>[4x]SMGPTSQRRGSLQLWQFLVALLDDPSNSHFIAWTGRGMEFKLIEPEEVARRWGIQKNRPAMNYDKLSRSLRYYYEKGIMQKVAGERYVYKFVCDPEALFSMAFSDN

The Ets transcription factor family consists of 28 genes in humans containing the evolutionarily conserved 85 amino acid Ets DNA-binding domain, originally identified as a viral oncogene (E26 transformation-specific). The Ets domain is a variant helix-turn-helix (winged helix) structure, comprising three α-helices and a four-stranded antiparallel β-sheet. Here, we present the crystal structures of the Ets domains of the entire PEA3 subfamily (Etv1, Etv4, and Etv5) together with the structure of the Erg family member (Fev). Furthermore, a new Ets dimerization interface linked by a redox-sensitive disulfide bond is identified, and this dimerization is shown to result in a significant inhibition of DNA binding, potentially linking Ets transcription factors with cellular redox regulatory mechanisms.

Crystals were obtained from constructs that contained the Ets domain, Etv1 (encompassing amino acids 326–429), Etv4 (encompassing amino acids 338–470), and Fev (encompassing amino acids 42–141). The construct of Etv1 included two inadvertent mutations that resulted from primer impurities as follows: Y329S at the N terminus, and P427S at the C terminus; this construct is denoted Etv1Y329S-P427S. Our attempts to crystallize the corresponding construct with the wild-type sequence failed, although the mutated residues are in disordered regions or at the end of the ordered region of the crystal structures of Etv1, so they are unlikely to have any bearing on the structural and functional analyses. Electron density is observed for residues Ser-334 to Phe-426 (thus excluding the Y329S and P427S mutations) with most side chains visible. We also compared the Etv-1 construct used for crystallization, which contains two primer-induced mutations, against wild-type Etv1 and found no significant difference in DNA binding. Etv1, Etv4, and Fev display the typical fold of the Ets domain, which contains three α-helices (α1–3) flanking a four-stranded β-sheet, with an additional C-terminal helix (α4). On an individual residue level, the most striking transitions can be seen to occur in the recognition helix α3, where in Etv1 Asp-387, Arg-391, and Arg-394 can be seen to become ordered upon DNA binding and Tyr-395, which can be seen to switch between the two alternative rotamers found to be important for recognition of bases downstream of the GGA motif in the Fev-DNA complex. Analysis of the contacts between adjacent molecules in the Etv1, Etv4, and Etv5 crystals reveals a conserved potential dimer interface that is distant from the DNA binding surface and is present in all the DNA-free and DNA-bound crystal forms. Dimerization of Etv1, -4, and -5 is mediated by the homologous cysteine residues (Cys-416, Cys-422, and Cys-449, respectively). The reduced monomeric Etv1 protein bound the DNA probe with an affinity up to 200-fold higher than the oxidized dimeric form; a C416S mutant of Etv1 bound DNA with an affinity similar to the reduced wild-type Etv1 (0.26 nm).> MAQVINTNSLSLLTQNNLNKSQSALGTAIERLSSGLRINSAKDDAAGQAIANRFTANIKGLTQASRNANDGISIAQTTEGALNEINNNLQRVRELAVQSANSTNSQSDLDSIQAEITQRLNEIDRVSGQTQFNGVKVLAQDNTLTIQVGANDGETIDIDLKQINSQTLGLDTLNVQQKYKVSDTAATVTGYADTTIALDNSTFKASATGLGGTDQKIDGDLKFDDTTGKYYAKVTVTGGTGKDGYYEVSVDKTNGEVTLAGGATSPLTGGLPATATEDVKNVQVANADLTEAKAALTAA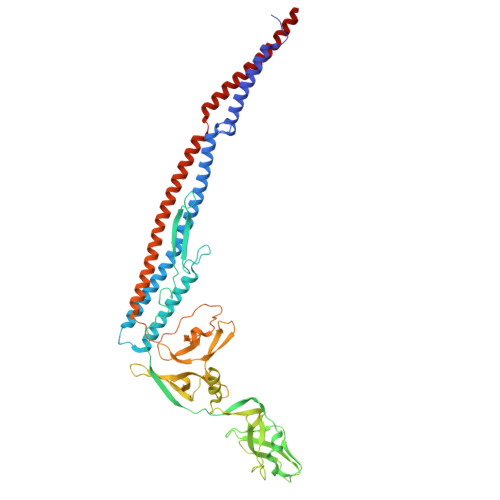GVTGTASVVKMSYTDNNGKTIDGGLAVKVGDDYYSATQNKDGSISINTTKYTADDGTSKTALNKLGGADGKTEVVSIGGKTYAASKAEGHNFKAQPDLAEAAATTTENPLQKIDAALAQVDTLRSDLGAVQNRFNSAITNLGNTVNNLTSARSRIEDSDYATEVSNMSRAQILQQAGTSVLAQANQVPQNVLSLLR>GPSREASNSATMFGFLVLGYLLYLVFGAVVFSSVELPYEDLLRQELRKLKRRFLEEHECLSEQQLEQFLGRVLEASNYGVSVLSQASGNWNWDFTSALFFASTVLSTTGYGHTVPLSDGGKAFCIIYSVIGIPFTLLFLTAVVQRITVHVTRRPVLYFHIRWGFSKQVVAIVHAVLLGFVTVSCFFFIPAAVFSVLEDDWNFLESFYFCFISLSTIGLGDYVPGEGYNQK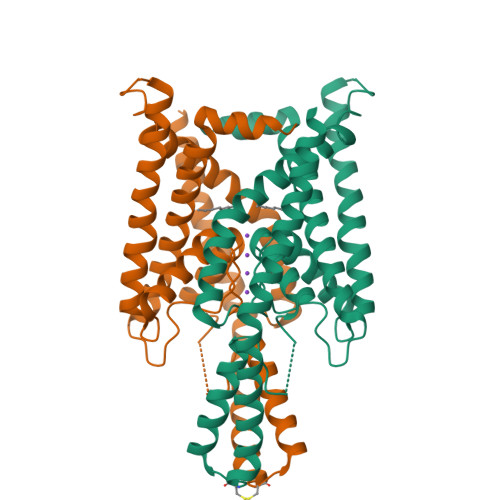FRELYKIGITCYLLLGLIAMLVVLETFCELHELKKFRKMFYVKKDKDEVD[4x]The sliding clamp is a ring-shaped protein complex that encircles DNA with the help of clamp loader in an ATP-dependent manner, and slides along the DNA. In prokaryotes, however, β-clamp is a homodimer, with each monomer consisting of three globular domains, and in this way β-clamp displays a six-domain ring. Although β-clamp is part of the DNA polymerase III holoenzyme, it is not attached to polymerase III permanently like the other subunits. β-clamp is loaded on the DNA, by clamp loader, a subunit of DNA Pol III. In both prokaryotes and eukaryotes, a key feature of this clamp-binding motif is the presence of hydrophobic amino acid residues that bind to the hydrophobic pocket in the C-terminal region of the clamp.

To validate the region in HpDNA ligase predicted by us to be an Hpβ-clamp binding region, we co-crystallized Hpβ-clamp with the peptide 554QEFIRSLF561 from DNA ligase. The co-crystal structure belongs to space group P212121 with four monomers making two dimers (first above the second) per asymmetric unit. Out of two dimers, the peptide was found to occupy both the binding sites of the first dimer, while second clamp dimer did not show any peptide bound to them. The binding of the peptide to the binding pocket of beta clamp is dominated by hydrophobic interactions. Out of eight residues of peptide 554QEFIRSLF561, the density for Gln554 and Glu555 was missing in both the chains. Ile557, Leu560 and Phe561 interact with the residues that are present in the cleft between domain II and III in both the chains suggesting their importance for β-clamp interaction. One noticeable thing is that residue Thr175 of β-clamp in both the chains makes hydrogen bond with backbone nitrogen of Leu560 from the peptide, suggesting that this must be a conserved residue in the protein-binding pocket. A comparison of the native β-clamp structure with the peptide-bound β-clamp structure showed differences in the positions of some of the residues at the protein-binding pocket of β-clamp. The residues involved in peptide binding reveal the maximal local displacement, the positions of residues Lys176 and M370 of β-clamp were found to differ between these two structures compared to native structure. The binding of ligase peptide at both interacting sites indicates that both sites of Hpβ-clamp could be used simultaneously as a processivity promoting factor.

>[4x]MAMKISVSKNDLENALRYLQAFLDKKDASSIASHIHLEVIKEKLFLKASDSDIGLKSYIFTQSSDKEGVGTINGKKFLDIISCLKDSNIILETKDDSLAIKQNKSSFKLPMFDADEFPEFPVIDPKVSIEVNAPFLVDAFKKIAPVIEQTSHKRELAGILMQFDQKHQTLSVVGTDTKRLSYTQLEKISIHSTEEDISCILPKRALLEILKLFYENFSFKSDGMLAVIENEMHTFFTKLIDGNYPDYQKILPKEYISSFTLGKEEFKESIKLCSSLSSTIKLTLEKNNALFESLDSEHSETAKTSVEIEKGLDIEKAFHLGVNAKFFLEALNALGTTQFVLRCNEPSSPFLIQESLDEKQSHLNAKISTLMMPITLELHHHHHH;>QEFIRSLF[2x]> MKTPLVTREGYEKLKQELNYLWREERPEVTKKVTWAASLGDRSENADYQYNKKRLREIDRRVRYLTKCMENLKIVDYSPQQEGKVFFGAWVEIENDDGVTHRFRIVGYDEIFGRKDYISIDSPMARALLKKEVGDLAVVNTPAGEASWYVN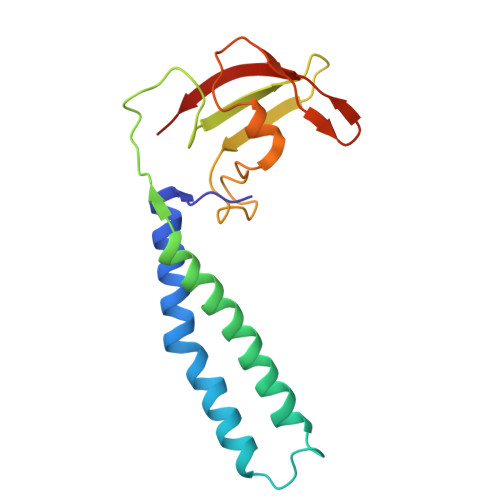AIEYVKP>[5x]GQDMVSPPPPIADEPLTVNTGIYLIECYSLDDKAETFKVNAFLSLSWKDRRLAFDPVRSGVRVKTYEPEAIWIPEIRFVNVQNARDADVVDISVSPDGTVQYLERFSARVLSPLDFRRYPFDSQTLHIYLIVRSVDTRNIVLAVDLEKVGKNDDVFLTGWDIESFTAVVKPANFALEDRLESKLDYQLRISRQYFSYIPNIILPMLFILFISWTAFWSTSYEANVTLVV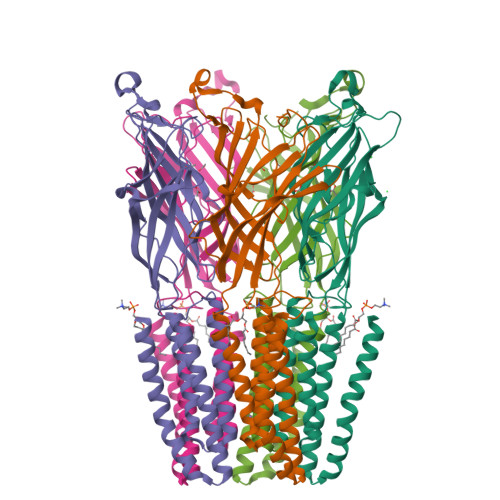STLIAHIAFNILVETNLPKTPYMTYTGAIIFMIYLFYFVAVIEVTVQHYLKVESQPARAASITRASRIAFPVVFLLANIILAFLFFGF>[2x]MKKENIISIQSQVFDGFCGNNIAAFVFRRRGHIPKILNTVQYYSKFKHSGVELNSQEVDIILSEYNKDQEFMNDSNIYFLTGYIKNAECVDMVTKNILELRRKRKIHRGKSNDNGNMNGHMNGHMNGHMNGHMNGHMNGHMNGHMNGHMNGHMNGHMNGHMNGHTNGHMNGHMNDHMNGHMN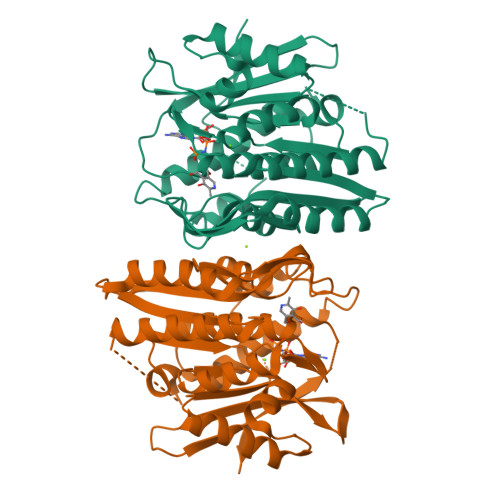GHTNDHMNGHTNDHMNGHTNDHMNGHTNDHMNDHMNGHTNDHMNDHMNDHMNGHTNSHTHGLTNGHMDEPNGEHPYRLMNSNELKSSHQIIPQGKQIHEKDMLKNNILTISQGRKKDEELYFIENIINLNFLWVCDPVMGDNGRLYVDERVVESYKKAIEYVDIITPNQYETELLCGIKINEEKDVIKCLDVLLHKGVKIVIITSVNYNFDKDHLFLYVSFFNNKNKIVYFKYKILKIHFNCFGSGDLFSCLLLSFIVKQKGNILHIISKVLNIVQNVIKNSLTGLELNIIENQDIIASDGLINDILIKEEPVFF>[2x]AESTLGAA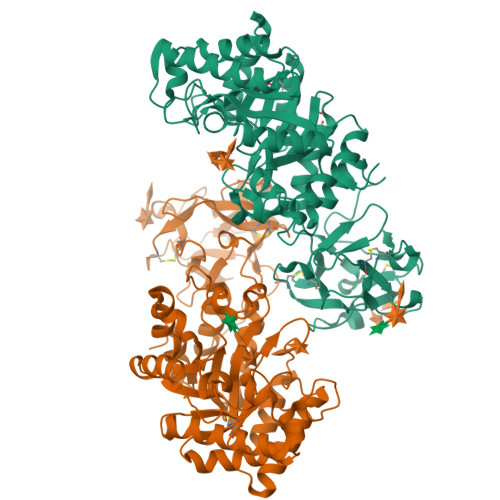AAQSGRYFGTAIASGKLGDSAYTTIASREFNMVTAENEMKIDATEPQRGQFNFSAGDRVYNWAVQNGKQVRGHTLAWHSQQPGWMQSLSGSTLRQAMIDHINGVMGHYKGKIAQWDVVNEAFSDDGSGGRRDSNLQRTGNDWIEVAFRTARAADPAAKLCYNDYNIENWTWAKTQGVYNMVRDFKQRGVPIDCVGFQSHFNSGSPYNSNFRTTLQNFAALGVDVAITELDIQGASSSTYAAVTNDCLAVSRCLGITVWGVRDTDSWRSGDTPLLFNGDGSKKAAYTAVLNALNGGSSTPPPSGGGQIKGVGSGRCLDVPNASTTDGTQVQLYDCHSATNQQWTYTDAGELRVYGDKCLDAAGTGNGTKVQIYSCWGGDNQKWRLNSDGSIVGVQSGLCLDAVGGGTANGTLIQLYSCSNGSNQRWTRT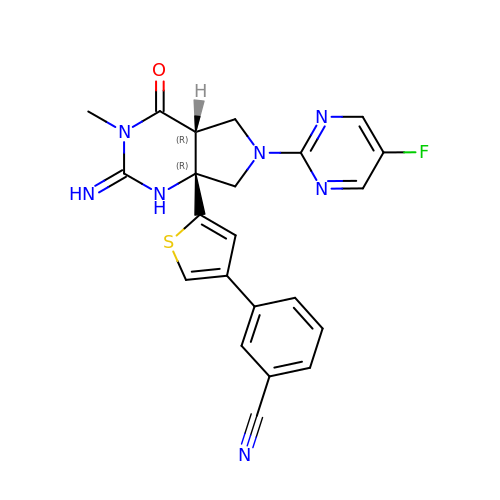3-{5-[(2E,4aR,7aR)-6-(5-fluoropyrimidin-2-yl)-2-imino-3-methyl-4-oxooctahydro-7aH-pyrrolo[3,4-d]pyrimidin-7a-yl]thiophen-3-yl}benzonitrile | C22 H18 F N7 O S | PTLJUNIICOHEHE-JTSKRJEESA-N>[2x]RGAEFTRLPVSWTVNPRDAANARAAWKTLSAYHRGKPKSSRKLHVVYVTFKDRPALEGYRERYDHILKNIQAYYADQMQANGFPPLTFQLDLDERGKLVIHDAYVDKPMSEMSVQSSGPVSREAARKVLASKGIDIEKEHVLVVCQLPDGVGPYYGGGFSHQGTGWTCDQEGLDPASFLDTEMMQGGRFKVTRGKNATIYIGGTAHELGHSFGLPHTGDGWNYPDAGASLMGHGNSTYG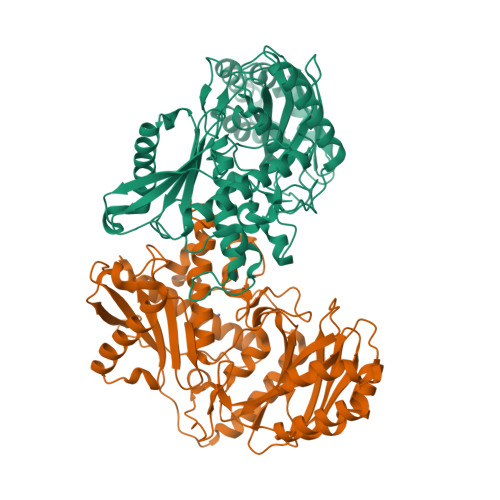DELRHEGKGAYLAPTDALKLASVPLFNGVETELPADASFGRMLGKYVPGSFERLEAIPVKDGLRLKGRVHLTRPAYGIVAHLDPPGGSDYDSNAVGASLDEKGEFDLTICRPGYKGGFIEMRVAVLNCDSTRSMITLPVWMDARGTKAPSLAQIVYFGDVQNLWIRGRTEEARKALAEVERRHGSRSEVKEWLPVWKRALGR S-Hydroxy-Glutathione | C10 H17 N3 O7 S | 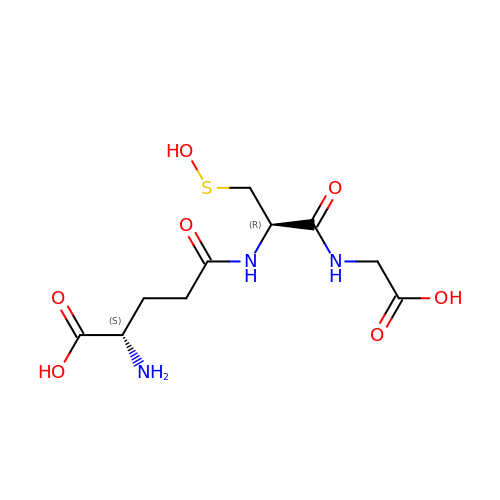PFXSQLOWBQWLCX-WDSKDSINSA-N>[2x]MCGIFAYLNYHVPR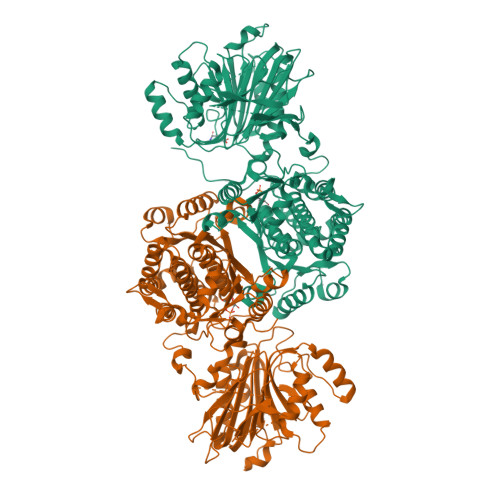TRREILETLIKGLQRLEYRGYDSAGVGFDGGNDKDWEANACKIQLIKKKGKVKALDEEVHKQQDMDLDIEFDVHLGIAHTRWATHGEPSPVNSHPQRSDKNNEFIVIHNGIITNYKDLKKFLESKGYDFESETDTETIAKLVKYMYDNRESQDTSFTTLVERVIQQLEGAFALVFKSVHFPGQAVGTRRGSPLLIGVRSEHKLSTDHIPILYRTGKDKKGSCNLSRVDSTTCLFPVEEKAVEYYFASDASAVIEHTNRVIFLEDDDVAAVVDGRLSIHRIKRTAGHHHHHHDHPGRAVQTLQMELQQIMKGNFSSFMQKEIFEQPESVVNTMRGRVNFDDYTVNLGGLKDHIKEIQRCRRLILIACGTSYHAGVATRQVLEELTELPVMVELASDFLDRNTPVFRDDVCFFLSQSGETADTLMGLRYCKERGALTVGITNTVGSSISRETDCEVHINAGPEIGVASTKAYTSQFVSLVMFALMMCDDRISMQERRKEIMLGLKRLPDLIKEVLSMDDEIQKLATELYHQKSVLIMGRGYHYATCLEGALKIKEITYMHSEGILAGELKHGPLALVDKLMPVIMIIMRDHTYAKCQNALQQVVARQGRPVVICDKEDTETIKNTKRTIKVPHSVDCLQGILSVIPLQLLAFHLAVLRGYDVDFPRNLAKSVTVE2-(4-HYDROXY-PHENYL)-CHROMAN-4-ONE | C15 H12 O3 | 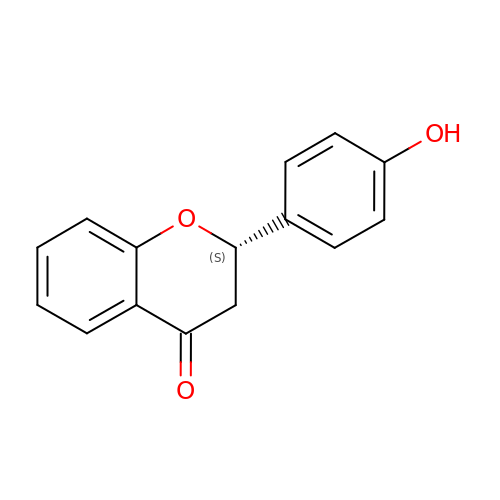ZLHVIYHWWQYJID-HNNXBMFYSA-N>MAEAEAGGDEARCVRLSAERAKLLLAEVDTLLFNCDGVLWRGETAVPGAPETLRALRARGKRLGFITNNSSKTRTAYAEKLRRLGFGGPVGPEAGLEVFGTAYCSALYLRQRLAGVPDPKAYVLGSPALAAELEAVGVTSVGVGPDVLHGDGPSDWLAVPLEPDVRAVVVGFDPHFSYMKLTKAVRYLQQPDCLLVGTNMDNRLPLENGRFIAGTGCLVRAVEMAAQRQADIIGKPSRFIFDCVSQEYGINPERT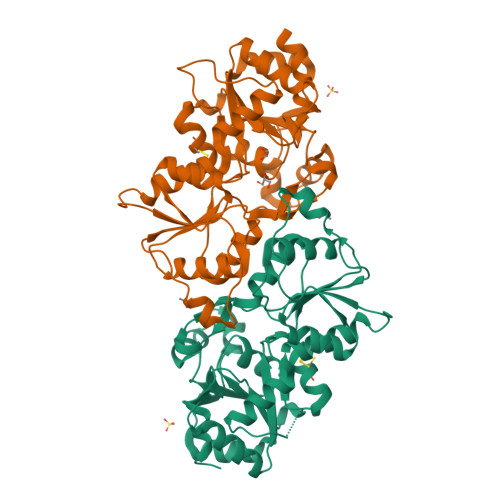VMVGDRLDTDILLGSTCSLKTILTLTGVSSLEDVKSNQESDSMFKKKMVPDFYVDSIADLLPALQG[8x]> MGKKAHGGKMKPEIDENGTLLVPPPRTIANQDHFHRLNYLYQISAYQTRARQKARTDAHTPLARNYIKSMDLISKKTKTSLLPTIKRTICKKC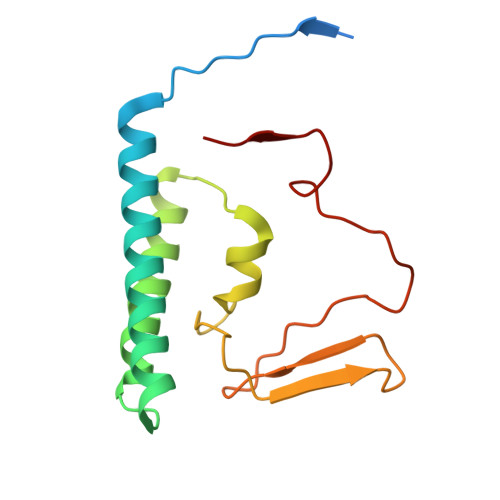HRLLWTPKKLEITSDGALSVMCGCGTVKRFNIGADPNYRTYSEREGNLLNS> MKFALQINEGPYQHQASDSAYQFAKAALEKGHEIFRVFFYHDGVNNSTRLTTPPQDDRHIVNRWAELAEQYELDMVVCVAAAQRRGIVDEGEASRNGKDATNIHPKFRISGLGQLVEAAIQADRLVVFGD;> MSEVVKKFMYLNRKAPYGTIYAWEALEVVLIGAAFDQDVCVLFLDDGVYQLTRGQDTKGIGMKNFSPTYRTLGDYEVRRIYVDRDSLEARGLTQDDLVEIAFEDMETEEEFDNIVE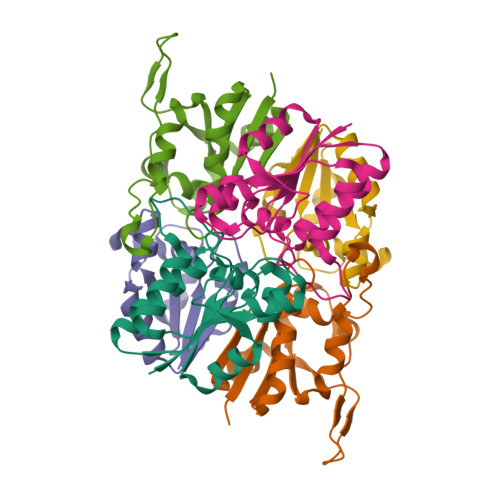VIDSARVSELMNESDAVFSF;> MSILHTVNKSPFERNSLESCLKFATEGASVLLFEDGIYAALAGTRVESQVTEALGKLKLYVLGPDLKARGFSDERVIPGISVVDYAGFVDLTTECDTVQAWL FtsEX comprises a cell division-regulating integral membrane protein (FtsX) and a cytoplasmic ATPase (FtsE) that resembles an ATP-binding cassette (ABC) transporter. Hydrolysis causes a conformational change that is transmitted through the membrane via FtsX, an integral membrane protein with two extracellular loops (ECLs), denoted the large (ECL1) and small (ECL2) loops. The folded structure (residues 57 to 166) reveals a central core composed of a four-stranded antiparallel β-sheet (β1, β6, β4, and β5) and two helices (α1 and α3), an α-helical lobe (residues 107 to 135) harboring the α2 helix, and an extended β-hairpin (β2 and β3). The helical lobe mediates a physical interaction with the peptidoglycan hydrolase PcsB via the coiled-coil domain of PcsB (PscBCC).

Three different structures, with resolutions ranging from 2.0 to 2.3 Å, were solved by X-ray crystallography, each in the presence of a different detergent. The detergents used were dodecyltrimethylammonium chloride (detergent 1 [D1]), n-undecyl-β-d-maltoside (detergent 2 [D2]), and n-decyl-β-d-maltoside (detergent 3 [D3]). In all cases, two independent protein molecules are present in the asymmetric unit, arranged in such a way as to keep hydrophobic residues from their α-helical lobes buried. Different conformations were observed for the β-hairpin and the helical lobe among the six structures, depending on the presence and identity of the detergent molecule bound to FtsXECL1. In any case, the crystal structures suggest that changes in the protein backbone and side chains of the helical lobe occur when a detergent ligand is bound. These changes create a cavity in which the detergent molecules insert, with a large part of the helical lobe (from Q111 to E127) affected by the interaction with detergent. Residues Y112, W123, E127, and F126 are strongly perturbed upon detergent ligand binding, with the hydroxyl moiety of Y112 interacting with carboxylate of E127. Changes in W123 and F126 stabilize the hydrophobic region of detergent 1. A similar interaction pattern is observed for detergents 2 and 3; additional interactions are observed in N131 with detergents 2 and 3, which are characterized by a larger hydrophilic head (maltose). Full stabilization of the hydrophobic tail of the detergents is completed by the same hydrophobic residues (W123 and F126) but from a symmetry-related molecule.

>TDIENNVRVVVYIRKDVEDNSQTIEKEGQTVTNNDYHKVYDSLKNMSTVKSVTFSSKEEQYEKLTEIMGDNWKIFEGDANPLYDAYIVEANAPNDVKTIAEDAKKIEGVSEVQD[2x]>GIDPFTGPHFVEYLSWEVTGECNVLLKCKVANIKKETHIVWYKDEREISVDEKHDFKDGICTLLITEFSKKDAGIYEVILKDDRGKDKSRLKLVDEAFKELMMEVCKKIALSATDLKIQSTAEGIQLYSFVTYYVEDLKVNWSHNGSAIRYSDRVKTGVTGEQIWLQINEPTPNDKGKYVMELFDGKTGHQKTVDLSGQAYDEAYAEFQRLKQAAIAEKNRARVLGGLPDVVTIQEGKALNLTCNVWGDPPPEVSWLKNEKALASDDHCNLKFEAGRTAYFT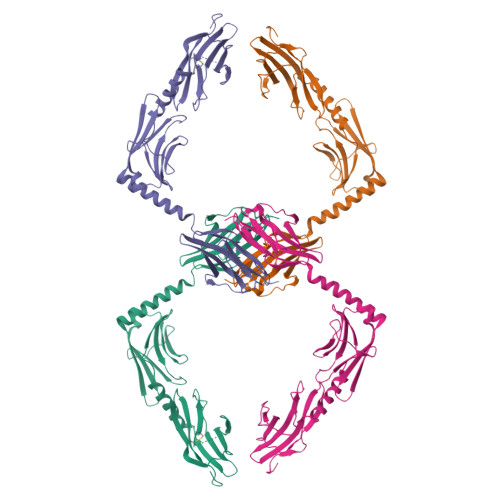INGVSTADSGKYGLVVKNKYGSETSDFTVSVFIPE[4x]N'-[6-[2-(6-AZANYL-4-METHYL-PYRIDIN-2-YL)ETHYL]PYRIDIN-2-YL]-N,N'-DIMETHYL-ETHANE-1,2-DIAMINE 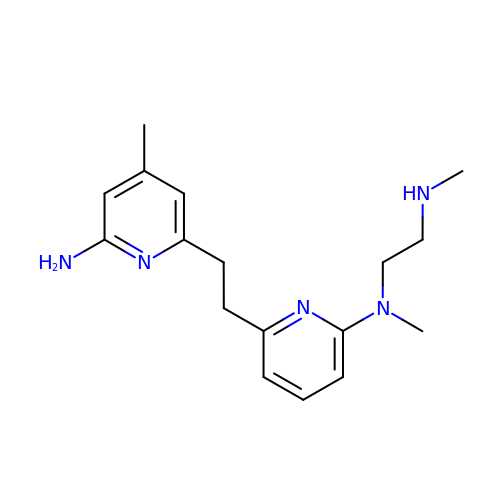| C17 H25 N5 | AVQUEPVPLWZPMB-UHFFFAOYSA-N> GPGSLSQASADLEATLRHKLTVMYSQINGASRALDDVRNRQQDVRMTANRK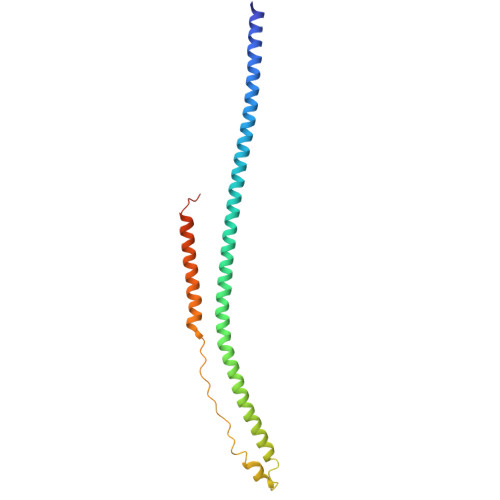VEQLQQEYTEMKALLDASETTSTRKIKEEEKRVNSKFDTIYQILLKKKSEIQTLKEEIEQSLTKRDEFEFLEKASKLRGISTKPVYIPEVELNHKLIKGIHQSTIDLKNELKQCIGRLQELTPSSGDPGEHDPASTHKSTRP>GYIVDMSKWNGSPDWDTAKGQLDLVIARVQDGSNYVDPVYKDYVAAMKARNIPFGSYAFCRFVSVEDAKVEARDFWNRGDKDSLFWVADVEVTTMSDMRAGTQAFIDELYRLGAKKVGLYVGHHKYEEFGAAQIKCDFTWIPRYGAKPAYPCDLWQYDEYGQVPGIG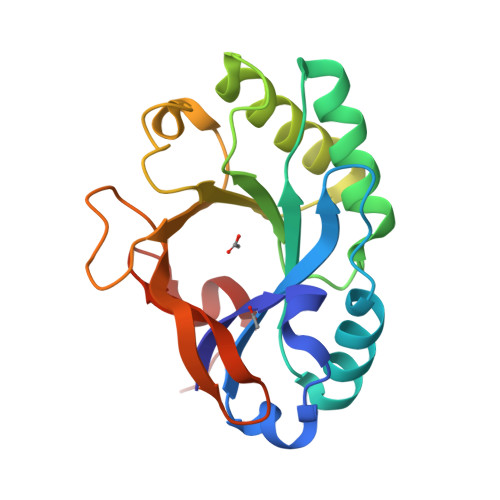KCDLNRLNGDKSLDWFTGKGEE[2x]>[2x]GNSVTYTTLISGLGKAGRLEEALELFEEMKEKGIVPNVVTYTTLISGLGKAGRLEEALELFEEMKEKGIVPNVVTYTTLISGLGKAGRLEEALELFEEMKEKGIVPNVVTYTTLISGLGKAGRLEEALELFEEMKEKGIVPNVVTYTTLISGLGKAGRLEEALELFEEMKE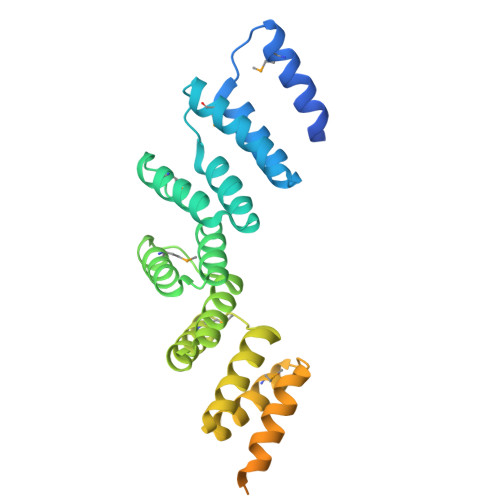KGIVPNVVTYTTLISGLGKAGRLEEALELFEEMKEKGIVPNVVTYTTLISGLGKAGRLEEALELFEEMKEKGIVPNVVTYTTLISGLGKAGRLEEALELFEEMKEKGIVPNVVTYTTLISGLGKAGCGRALE> TILRQLLPKNRRVTSGRRTT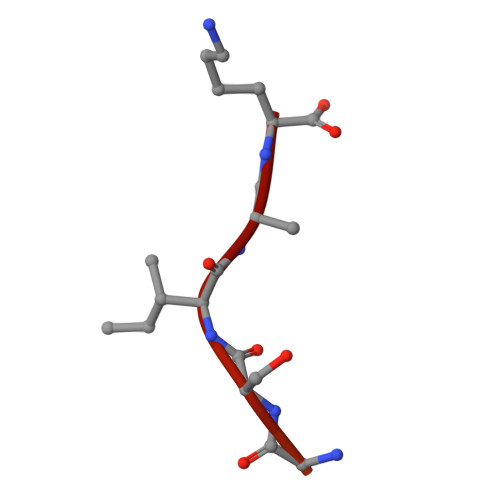SAAGGIRKISGSIKK> GAMDRLRAAEHPRPDYVLLHISDTHLIGGDRRLYGAVDADDRLGELLEQLNQSGLRPDAIVFTGDLADKGEPAAYRKLRGLVEPFAAQLGAELVWVMGNHDDRAELRKFLLDEAPSMAPLDRVCMIDGLRIIVLDTSVPG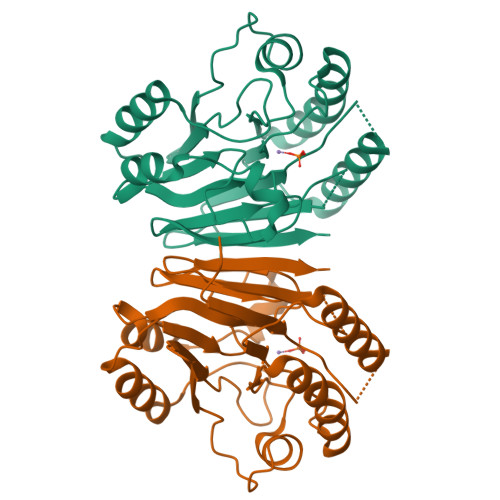HHHGEIRASQLGWLAEELATPAPDGTILALHHPPIPSVLDMAVTVELRDQAALGRVLRGTDVRAILAGHLHYSTNATFVGIPVSVASATCYTQDLTVAAGGTRGRDGAQGCNLVHVYPDTVVHSVIPLGGGETVGTFVSP> SAPADYFRILVQQFEVQLQQYRQQIEELENHLATQANNS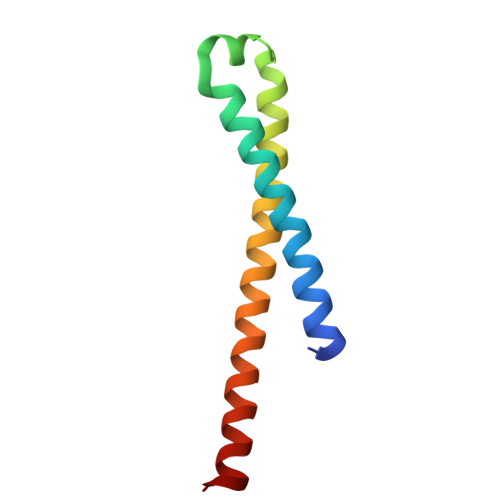HITPQDLSMAMQKIYQTFVALAAQLQSIHENVKVLKEQYLGYRKMFLG> MPVDFTGYWKMLVNENFEEYLRALDVNVALRKIANLLKPDKEIVQDGDHMIIRTLSTFRNYIMDFQVGKEFEEDLTGIDDRKCMTTVSWDGDKLQCVQKGEKEGRGWTLWIEGD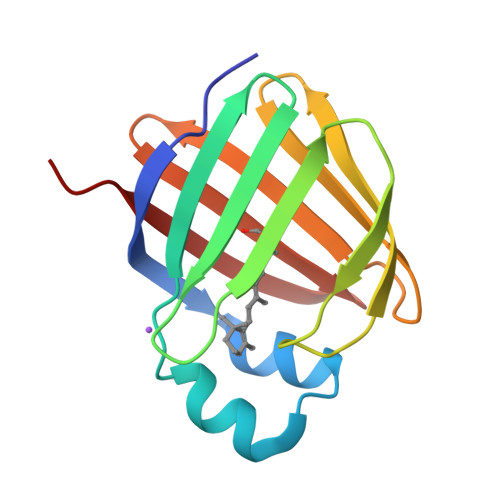ELHLEMRVEGVVCKQVFKKVQ Zandelisib | C31 H38 F2 N8 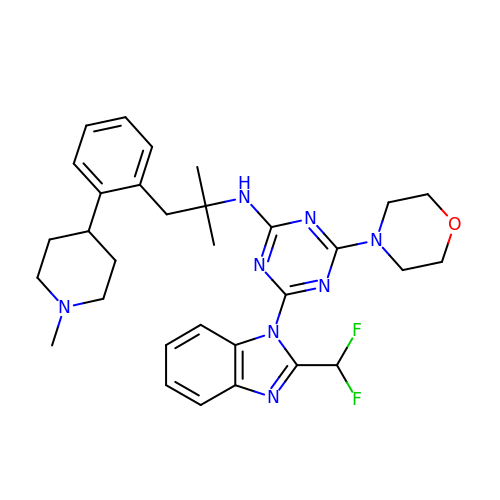O | WPFUFWIHMYZXSF-UHFFFAOYSA-N> WSAEDKHKEGVNSHLWIVNRAIDIMSRNTTLVKQDRVAQLNEWRTELENGIYAANYENPYYDNSTFASHFYDPDNGKTYIPFAKQAKETGAKYFKLAGESYKNKDMKQAFFYLGLSLHYLGDVNQPMHAANFTNLSYPQGFHSKYENFVDTIKDNYKVTDGNGYWNWKGTNPEEWIHGAAVVAKQDYSGIVNDNTKDWFVKAAVSQEYADKWRAEVTPMTGKR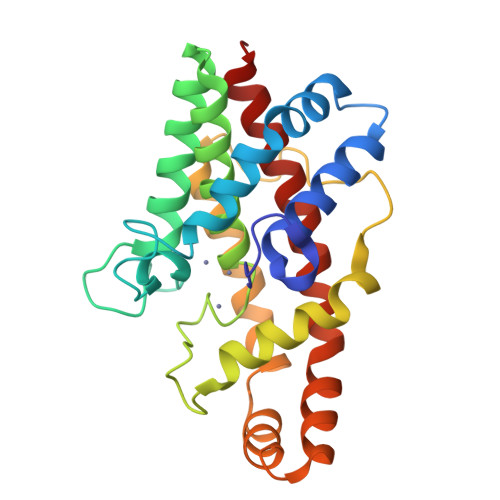LMDAQRVTAGYIQLWFDTYGDR>[5x]LTDLTKNEKGRLTPITKQQSANSAKLTAYGTLKSALEKFQTANTALNKADLFKSTVASSTTEDLKVSTTAGAAAGTYKINVTQLAAAQSLATKTTFATTKEQLGDTSVTSRTIK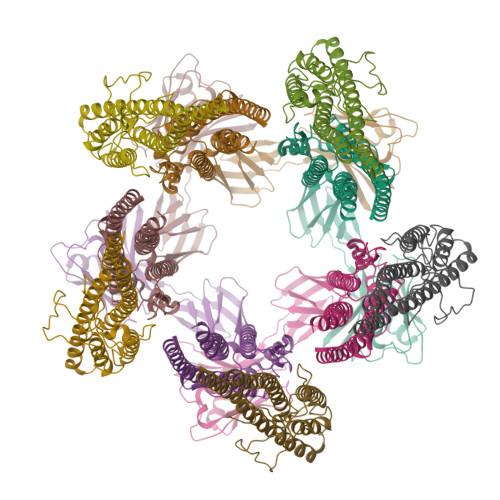IEQPGRKEPLEIKLDKGDTSMEAIRDAINDADSGIAASIVKVKENEFQLVLTANSGTDNTMKITVEGDTKLNDLLAYDSTTNTGNMQELVKAENAKLNVNGIDIERQSNTVTDAPQGITLTLTKKVTDATVTVTKDDTKAKEAIKSWVDAYNSLVDTFSSLTKYTAVEPGEEASDKNGALLGDSVVRTIQTGIRAQFANSGSNSAFKTMAEIGITQDGTSGKLKIDDDKLTKVLKDNTAAARELLVGDGKETGITTKIATEVKSYLADDGIIDNAQDNVNATLKSLTKQYLSVSNSIDETV;>VLSQAQAQNSQYALARTFATQKVSLEESVLSQVTTAIQTAQEKIVYAGNGTLSDDDRASLATDLQGIRDQLMNLANSTDGNGRYIFAGYKTEAAPFDQATGGYHGGEKSVTQQVDSARTMVIGHTGAQIFNSITSNAVPEPDGSDSEKNLFVMLDTAIAALKTPVEGNNVEKEKAAAAIDKTNRGLKNSLNNVLTVRAELGTQLSELSTLDSLGSDRALGQKL[5x]>MTSRIRFLMCPPDHYDVDYVINPWMEGNIHKSSRDRAVEQWQGLYQILKEHAIVDLVTPQKGWPDLVFTANAGLVLGDNVVLSRFLHKERQGEEP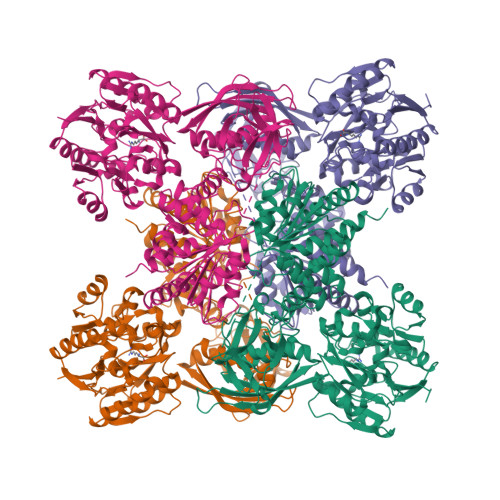YFKEWFEGNGYTVYELPKDLPFEGAGDALLDREGRWLWAGYGFRSELDSHPYLAKWLDIEVLSLRLIDERFYHLDTCFCPLANGYLLYYPGAFDSYSNRLIEMRVAPEKRIAIAEADAVNFACNTVNVESIVIMNKASDALKQSLTGVGFQVLETPLTEFLKAGGAAKALTLRVTEPVRDEVHANVYVESRIIRIEGHLLDSGLINRALDMIVDTGGSFQVLNFNLGEQRQSTSAAEVKVSAPSHEVMEEIISLLIDLGAVDLPQDERDAKLEPVIQDGVAPDDFYVSTIYPTEVRINGQWIKVENQRMDGAIAITQTPNGLLAQCKILRDLKAGEQVIVDVLGIRTIRKTESREQRNTQEFSFMSGGVSSERRVELVVEQVAWELRKIRDAGGKVVVTAGPVVIHTGGGEHLSRLIREGYVQALLGGNAIAVHDIEQNMMGTSLGVDMKRGVAVRGGHRHHLKVINTIRRHGSIAKGVESGIIRSGVMYECVRNQIPFVLAGSIRDDGPLPDTQMDLIKAQEEYAKHLEGAEMILMLSSMLHSIGVGNMTPAGVKMVCVDINPAVVTKLSDRGSIESVGVVTDVGLFLSLLTQQLDKLTSPYVSKVG[2x]5-{4-[3-(2-methoxypyrimidin-5-yl)phenyl]piperazin-1-yl}pyrimidine-2,4-diamine | C19 H22 N8 O | 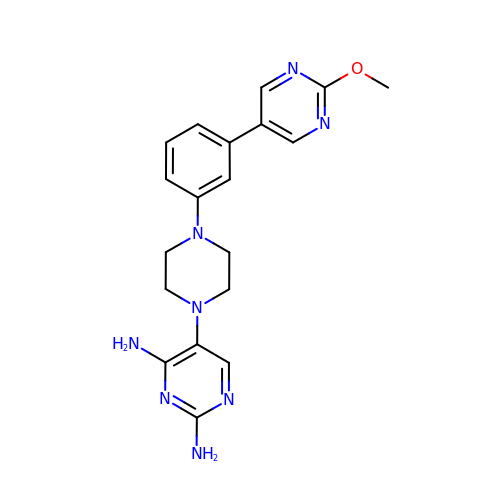GUZBZPCNAJDYMO-UHFFFAOYSA-N>[5x]SNAMIIRPEQHWFLRLFDWHASVLSKIIFRLLLNVLMSIIAIISYQWYEQLGIHLTVAPFSLLGIAIAIFLGFRNSASYSRFVEARNLWGTVLIAERTLVRQLRNILPAEHDAHRRIVSYLVAFSWSLKHQLRKTDPTADLRRLLPEERVTEILASSMPTNRILLLAGNEIGQLREAGKLSDITYGLMDNKLDELAHVLGGCERLATTPVPFAYTLILQRTVYLFCTLLPFALVGDLHYMTPFVSVF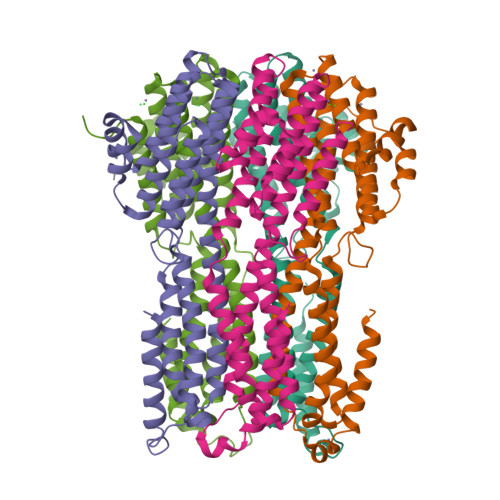ISYTFLSWDSLAEELEDPFGTAANDLPLNAMCNTIERNLLDMTGQHPLPE> TTNTDSFTFSKFKPNQPNLKKQGDATVTSSGTLQ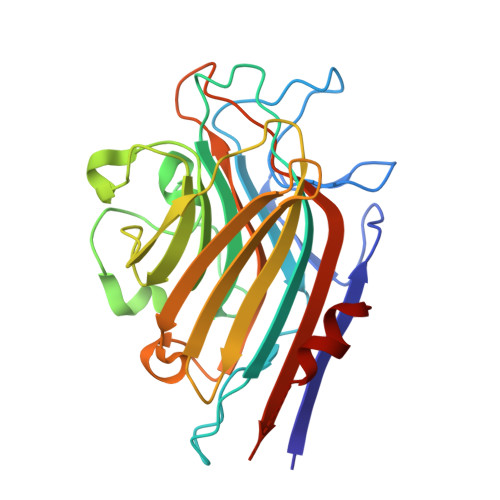LTKVDKNGVPDPKSLGRALYASPINIWDSKTGVVASFATSFRFTIYAPNIATIADGLAFFLAPVSSPPKAGAGFLGLFDSAVFNSSYQTVAVEFDTYENTVFLDPPDTHIGIDVNSIKSIKTVKWDLANGEAAKVLITYDSSAKLLVAALVYPSSKTSFILSDVVDLKSVLPEWVSIGFSAATGASSGYIETHDVFSWSFASKLSFXXXXXXLDLASFLVAN> SSSNYCNQMMKSRNLTKDRCKPVNTFVHESLADVQAVCSQKNVACKNGQTNCYQSYSTMSITDCRETGSSKYPNCAYKT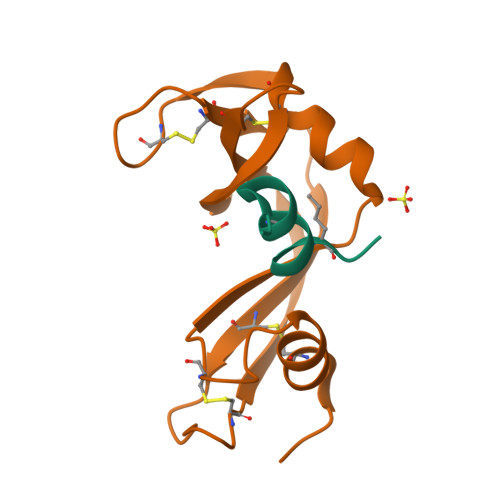TQANKHIIVACEGNPYVPVHFDASV;> KETAAAKAERQHLDS>GPLGSSRLYLQNTAVMEELYRRNLSEDLVRDNGLSCGGREYWREPASTVGAASDGLSEEERRTAADAAERMTAVIAGTPGIAVERNVRDFRRGGWDVTPDNVESEFREVERRTFSDGVHWGRVIAFLAFSMSFAAYVNSRGIDGGAYSVFNWTLRVLNDSLADFIQRENGWRGFIVYADTLLRAQGS[2x];>[2x]ASSMASEVGRRLAEFGDQVDGQFYQ

A critical group of proteins that regulate apoptosis are the B-cell lymphoma-2 (Bcl-2) family and these proteins regulate intrinsic (mitochondrial-mediated) apoptosis. The sponge Geodia cydonium expresses a putative pro-survival Bcl-2 homolog, BHP2, that protects sponge tissue against apoptosis induced by heat-shock or tributylin (an organic tin derivative) exposure, as well as mammalian Hek-293 and NIH-3T3 cells against serum withdrawal or tributylin. To elucidate molecular mechanisms of apoptosis in these early lifeforms we have performed structural and binding studies on BHP2 and LB-Bak-2 from G. cydonium and L. baicalensis, respectively. We demonstrate that BHP2 shares the Bcl-2 fold with its higher organisms and, like them, bears a binding groove that binds the BH3-region of LB-Bak-2.

The structural basis for BH3 motif binding by BHP2, and its ability to discriminate against human pro-apoptotic Bcl-2 proteins over their sponge counterparts, was determined by solving the crystal structure of BHP2 bound to the LB-Bak-2 BH3 motif. Like other Bcl-2 orthologs BHP2 adopts a globular helical bundle fold comprising 8 α-helices, with helices 2–5 forming the canonical binding groove observed in all other pro-survival Bcl-2 family members. Clear and continuous electron density is observed for residues 18–38 and 67–198, with the intervening linker region being largely disordered except for a short helical turn formed by residues 53–57 that anchor the loop to the solvent exposed side of helix 6 from the main globular motif. Similar to pro-survival Bcl-2 proteins from higher organisms, BHP2 engages the LB-Bak-2 BH3 motif via the canonical Bcl-2 binding groove formed by α-helices 2–5. A total of 913 Å2 of solvent accessible surface is buried in the process. As expected, BHP2 Arg135BHP2 from the conserved BH1 motif forms an ionic interaction with the LB-Bak-2 Asp80Bak, an interaction conserved in almost all Bcl-2-BH3 motif interactions. Interestingly, Asp80Bak is also engaged in a second ionic interaction with His132BHP2, which in turn also contacts Asp83Bak, leading to the formation of a network of ionic interactions centering on LB-Bak-2 Asp80. A hallmark of pro-survival Bcl-2:pro-apoptotic BH3 motif interactions is the engagement of four highly conserved hydrophobic residues from the BH3 motif by the ligand binding groove of pro-survival Bcl-2.7 While BHP2 accommodates V71, L75 and V82, unexpectedly F78 is not captured by a hydrophobic pocket at the floor of the binding grove. Instead, the helical turn in LB-Bak-2 BH3 that features F78 is bulged out, allowing F78 to sit on top of BHP2 I94. This shift is enforced by the positioning of I94 in BHP2, where the protruding Ile side chain prevents access of LB-Bak-2 F78 into the typical position adopted in other pro-survival Bcl-2:BH3 motif complexes.> MNLIPTVIEQTSRGERAYDIYSRLL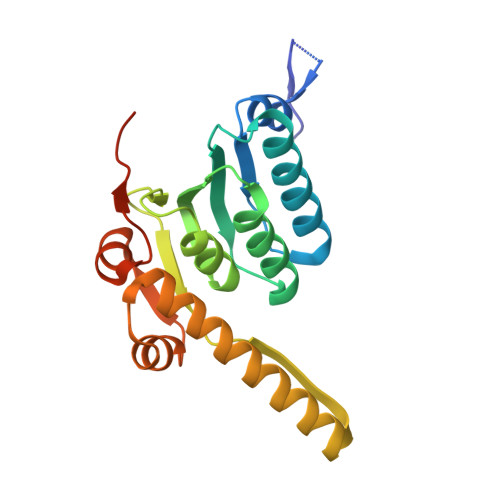KDRIIMLGSAIDDNVANSIVSQLLFLDAQDPEKDIFLYINSPGGSISAGMAIYDTMNFVKADVQTIGMGMAASMGSFLLTAGANGKRFALPNAEIMIHQPLGGAQGQATEIEIAARHILKIKERMNTIMAEKTGQPYEVIARDTDRDNFMTAQEAKDYGLIDDIIINKSGLKGHHHHHH>[4x]VT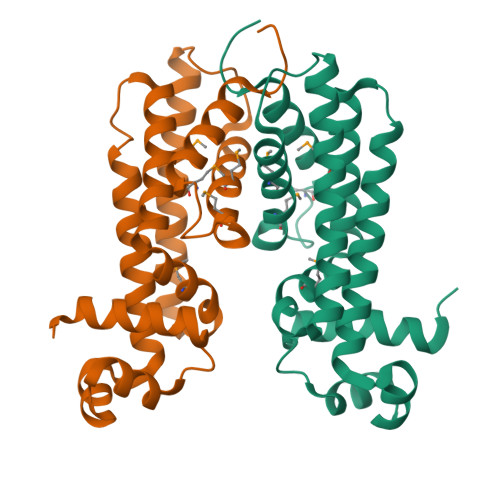TTRDRILEEAAKLFTEKGYEATSVQDLAQALGLSKAALYHHFGSKEEILYEISLLALKGLVAAGEKALEVADPKEALRRFMEAHARYFEENYPFFVTMLQGIKSLSPENRLKTIALRDRHEENLRAILRRGVEQGVFREVDVALAGRAVLSMLNWMIRWFRPDGPMRAEEVARAYHDLILRGLERGSA>AMADLEQKVLEMEASTYDGVFIWKISDFPRKRQEAVAGRIPAIFSPAFYTSRYGYKMCLRIYLNGDGTGRGTHLSLFFVVMKGPNDALLRWPFNQKVTLMLLDQNNREHVIDAFRPDVTS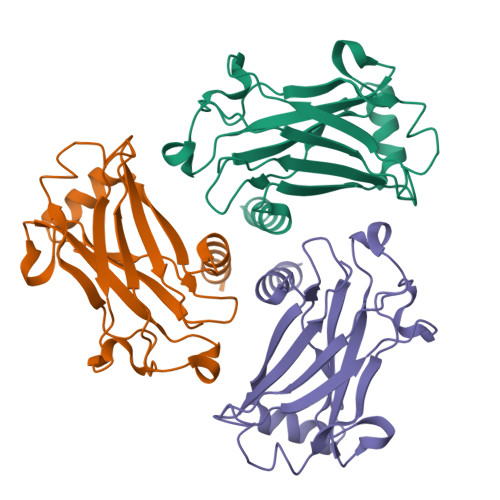SSFQRPVNDMNIASGCPLFCPVSKMEAKNSYVRDDAIFIKAIVDLTGL[6x];>XMLSVEEEG[3x]> GPMETTNWIGDENLTGNAEAPAKDDVVPDKNQFRYQKEELAAFCHFGPNTFNEIEWGEHYGNQKPSEIFTLKNDFDAETLVKTLKDAGFKKLIVTAKHHDGFCIWDSEHTEYDVKASGYKNKNGESDILAEISKACTDQNMDMGLYLSPWDIHEPSYGYKDEHGNPTTPDKDAKDYNEFYNNQLEEILGNPKYGNDGHFVEVWMDGAKGSGANAQEYDFKKWFKTIQDNEGKAAGYDADCMLFGAEAYTTVRWIGNELGIAGKDTWSKSKVDKDKNTINSNKQGNATVGFEDGDQWTVPEADARITSGWFWGTKKNTPKTMEELSDMYFNSVGHNATLLLNVPPNNQGTVDKAILDRVTEFGNNIKATFKTNLAKAEGASVKVSEVRGGAKEYKPGNMIDDNDETYWATSDGKKSGEILIDLGKETKFDVVSIEEAIQNGQRINNYKVEYRNGDSGTWTLLEEGKTIGAKRLCRTSETTARQIKITVGTCDGKVPMISEIGVYKSTEDMEKPNPIPKGMEVIDVEDKDVADGKGFTFKGKWNPENQPQYING

To access this source of nutrients, gut bacteria encode α-l-fucosidases (fucosidases) which catalyze the hydrolysis of terminal α-l-fucosidic linkages. We identified and characterized a fucosidase from R. gnavus E1 with the capacity to recognize fucosylated glycans capped with sialic acid and to hydrolyze α1–3/4 fucosyl linkages in these substrates without the need to remove sialic acid. The enzymatic characterization of R. gnavus fucosidases focused on previously uncharacterized bacterial fucosidases revealed that fucosidase ATCC_03833 belongs to GH29-A while E1_10125 belongs to GH29-B subfamily. The enzyme consists of two distinct domains, a catalytic domain (PF001120) domain comprising residues 46–366 in N-terminal and a F5/8 Type C domain (PF00754) covering residues 385–526 in C-terminal.

To further investigate E1_10125 ligand specificity, the enzyme was crystallized in the presence of 2′FL, providing the crystal structure of the complex showing the β-fucose anomer bound in the active site. Electron density maps allowed modelling of residues 23–527. The catalytic machinery sits in a cleft in the center of the N-terminal domain. By proximity to the bound fucose residue and homology to other fucosidases, Asp221 was identified as the catalytic nucleophile and Glu273 as the acid/base (amino acid numbering based on recombinant protein sequence). Trp325 creates a CH–π interaction with the bound ligand and His61, Trp72, His114, His115 and Tyr162 provides additional hydrogen bonding interactions. Phe59 and Trp219 provide a hydrophobic pocket to accommodate the fucose C6 methyl group. The fucose binding site is conserved with the S. pneumoniae and B. longum GH29 fucosidases and is henceforth referred to as the − 1 subsite. In the E1_10125 crystal structure, adjacent to the proposed + 2 site is an open platform comprises primarily neutral and hydrophobic residues, which would accommodate Neu5Ac. This is in marked contrast to the S. pneumoniae and B. longum homologue structures where this region is partially occluded by incoming loops. The ability to accommodate the sialic acid moiety, as also confirmed by STD NMR, appears to be enabled by an open region adjacent to the + 2 site (Gal residue in Le antigens), which  comprises residues Met220, Phe259, Gly260, Ala261 and Thr265 with additional stabilizing interactions likely to be provided by Trp269 and Glu262.>SKSTAEIRQAFLDFFHSKGHQVVASSSLVPHNDPTLLFTNAGMNQFKDVFLGLDKRNYSRATTSQRCVRAGGKHNDLENVGYTARHHTFFEMLGNFSFGDYFKLDAILFAWLLLTSEKWFALPKERLWVTVYESDDEAYEIWEKEVGIPRERIIRIGDNKGAPYASDNFWQMGDTGPCGPCTEIFYDHGDHIWGGPPGSPEEDGDRYIEIWNIVFMQFNRQADGTMEPLPKPSVDTAMGLERIAAVLQHVNSNYDIDLFRTLIQAVAKVTGAT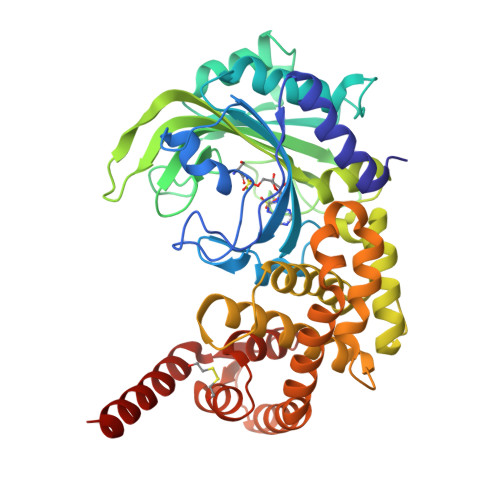DLSNKSLRVIADHIRSCAFLIADGVMPSNENRGYVLRRIIRRAVRHGNMLGAKETFFYKLVGPLIDVMGSAGEDLKRQQAQVEQVLKTEEEQFARTLERGLALLDEELAKLSGDTLDGETAFRLYDTYGFPVDLTADVCRERNIKVDEAGFEAAMEEQRRRAREASGF[2x]> ETGDQFSPNCSAVTHIFQARGIDAIEIPQKPSNERVLRYCESPSVGTCCTYNMETRMAMQSRQQLEGHTKDQISRMSGILGSKATKFKDIFTALLKESRTQFNSMFIRTYGVIYERNSYVFSDLFKELETYFANGRVDLLEVMDKFFNTLYQKMFTVLNTQYTFDENYMRCVSEHMKELKPFGDVPDKLSVQIKRSFVATRTYGQALTTASEVAKKVLNVRLNADCTGALTKMQHCGACKGYTEKPCTNYCVNVIKGCLHYQHEFDSEWENFAMAMDKVAERLLGSFNIVMVVEPLNIKISEAIMNFQDSGQDITNRVFQGCGRPKLQAMKQSISPKLQGVQILNARSPVEADTLDIDET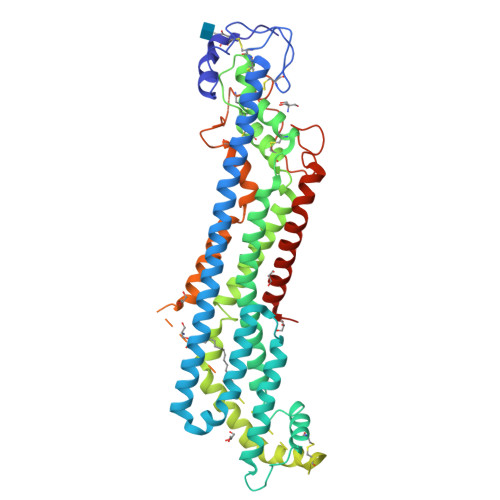LDEAIVLQERAAAEPGSQETSAQQSQEQGVGKSGNGGGGGGGNNRRQQQRRKQQQQRRKQQNNRDDNDDDDNESGGGREPILDRIVRDIRQRVKDYKKFWSNLPHSVCSNEDIASSSDVDGMCWNGHTIDRYMHSITTEHGSNPEFTGNPASTKQTAQMASQLSHLKNAIVHLRNAYNGQDVEWSEQGTLEVLFQ The proteins in the PIN-FORMED (PIN) family (also known as the auxin efflux carrier family) are key participants in this process and control auxin export from the cytosol to the extracellular space. PIN8 is a non-canonical PIN of 40 kDa in size, with a short cytosolic loop of 43 residues that lacks the phosphorylation motifs seen in the long auto-inhibitory loops of canonical PINs. The structure forms a homodimer, with each monomer divided into a transport and scaffold domain with a clearly defined auxin binding site. The structures and biochemical data reveal an elevator-type transport mechanism reminiscent of bile acid/sodium symporters, bicarbonate/sodium symporters and sodium/proton antiporters.

We solved three distinct structures of PIN8 using single-particle cryo-EM after reconstitution of the purified protein into peptidisc: an apo form at 2.9 Å resolution, PIN8 with IAA bound at 3.2 Å, and PIN8 with NPA bound at 3.4 Å resolution. The apo form of PIN8 displays a symmetric dimer of PIN8 characterized by a twofold rotation axis perpendicular to the membrane plane with a distinct concavity extending into the membrane along this axis from the non-cytosolic side. The scaffold domain comprises helices M1, M2, M6 and M7 and creates a large interface (1,512 Å2) to the other monomer in the dimeric complex. This interface is mediated mainly by M2 and M7, and is further stabilized by a lipid in a groove between M1 and the kinked M6. We also observe another lipid with an aliphatic tail sticking into a pocket of the transporter domain. Next to the crossover, there is a well-defined water-filled binding pocket nestled between the scaffold domain and the transporter domain that is open to the non-cytosolic side of the protein via the concavity. By contrast, access to the cytosol is blocked, clearly defining the conformation of the apo-PIN8 dimer as an empty outward-open state. The higher-resolution apo-PIN8 map reveals two peaks in the site, which are modelled as water. The highest-resolution map of the apo form was used for initial model building, but all maps display excellent density for the entire protein except for 39 residues of the disordered cytosolic loop, which were not modelled.

>[2x]MGISWLDIYHVVSATVPLYVSMTLGFLSARHLKLFSPEQCAGINKFVAKFSIPLLSFQIISENNPFKMSPKLILSDILQKFLVVVVLAMVLRFWHPTGGRGGKLGWVITGLSISVLPNTLILGMPILSAIYGDEAASILEQIVVLQSLIWYTILLFLFELNAARALPSSGASLEHTGNDQEEANIEDEPKEEEDEEEVAIVRTRSVGTMKILLKAWRKLIINPNTYATLIGIIWATLHFRLGWNLPEMIDKSIHLLSDGGLGMAMFSLGLFMASQSSIIACGTKMAIITMLLKFVLGPALMIASAYCIRLKSTLFKVAILQAALPQGVVPFVFAKEYNLHPEIISTGVIFGMLIALPTTLAYYFLLDLPGENLYFQ(3R)-3-methyl-4-[3-(1H-tetrazol-5-yl)phenoxy]-2,3-dihydrofuro[2,3-f]quinazoline-7,9-diamine 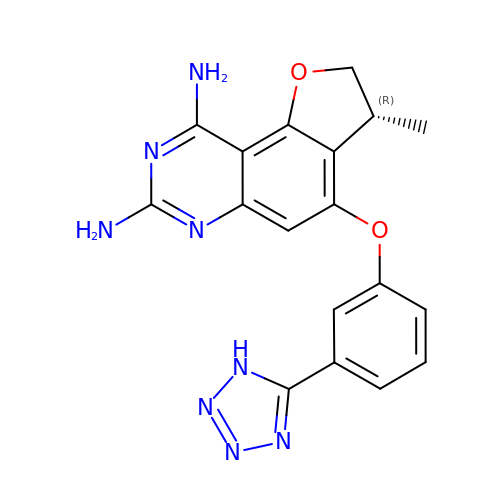| C18 H16 N8 O2 | HXCFGIFBIXRFOX-QMMMGPOBSA-N> GSEEVVQDAPLENNELNAEIDLQKTIQEEYKLWKQNVPFLYDLVITHALEWPSLTIQWLPDKKTIPGTDYSIQRLILGTHTSGNDQNYLQIASVQLPNFDEDTTEFTPSTIRRAQATGSYTIEISQKIPHDGDVNRARYMPQKPEIIATMGEGGNAYIFDTTCHDALTTGEALPQAVLKGHTAEGFGLCWNPNLPGNLATGAEDQVICLWDVQTQSFTSSETKVISPIAKYHRHTDIVN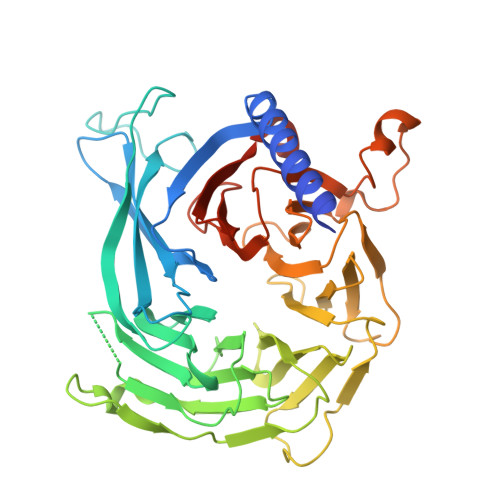DVQFHPQHEALLASVSDDCTLQIHDTRLNPEEEAPKVIQAHSKAINAVAINPFNDYLLATASADKTVALWDLRNPYQRLHTLEGHEDEVYGLEWSPHDEPILASSSTDRRVCIWDLEKIGEEQTPEDAEDGSPELLFMHGGHTNRISEFSWCPNERWVVGSLADDNILQIWSPSRVIWGRDHVQVSPRDLE CA forms the capsid shell surrounding the viral core that protects and transports the viral genome and also interacts with host cell factors that are necessary for trafficking, nuclear entry and proviral integration. Further, we assemble particles from HML2 CArec in vitro and use single-particle cryogenic electron microscopy (cryo-EM) to determine the high-resolution structures of four different types of Fullerene shell assemblies. Our studies of HML2 CArec show that an ERV retains the ability to form capsid assemblies using the same architecture as exogenous viruses. Analysis of the shell structures reveals the intra- and inter-molecular interactions that drives CA assembly into pentamers and hexamers and their association into shells that encapsidate the retroviral genome.

The D6 particles are also capsular with fully six-fold symmetric hexamers at the poles each surrounded by a ring of six pentamers and with six equatorial hexamers with similar distortions to those observed in the D5 structure. However, a comparison of the pentamer with the D6 polar hexamer, which obeys strict six-fold symmetry, shows that although helix α1–α2–α3 packing is maintained, in hexamers, the CArec monomers are positioned at a greater radius and are rotated away from the symmetry axis, relative to pentamers. As a result, the relative tilt angle between adjacent α1 helices is reduced and helix α2 comes closer to α3 of the neighbouring monomer allowing the additional monomer to be accommodated into the hexameric ring. In the D6 hexamer, because of the expanded radius, for the CTD to maintain the interaction with the neighbouring NTD it is rotated by a further 15° and there is an accompanying 2 Å shift and tilt between α6 and α7. This results in an alternative hydrogen-bonding configuration that defines the hexamer conformation where R143 now makes an intra-monomer hydrogen bond with the side chain of Q181 on the penultimate turn of α7, D171 is hydrogen bonded with S79′ but with a shifted geometry and the K229-D90′ interaction is absent. Moreover, adaptation of hexamers to the local environment is also a feature of our other D5 and D6 capsular assemblies, where hexamers interact with each other in the equatorial belt. Again, the pentamer conformation remains invariant and the hexamer six-fold symmetry is broken by NTD domain movements, changes in the NTD–CTD linker conformation and in the intra-hexamer CTD–NTD hydrogen bonding configuration and in the CTD radial position when interacting with either a neighbouring pentamer or hexamer. In the D5 and D6 particles, further configurations are possible depending on whether pentamers and hexamers are located at poles or are equatorial and interact either longitudinally or laterally.

>PVTLEPMPPGEGAQEGEPPTVEARYKSFSIKMLKDMKEGVKQYGPNSPYMRTLLDSIAHGHRLIPYDWEILAKSSLSPSQFLQFKTWWIDGVQEQVRRNRAANPPVNIDADQLLGIGQNWSTISQQALMQNEAIEQVRAICLRAWEKIQDPGSACPSFNTVRQGSKEPYPDFVARLQDVAQKSIADEKARKVIVELMAYENANPECQSAIKPLKGKVPAGSDVISEYVKACDGIGGAMHKAMLMAQLE[9x]>EKVIIEKAAGDAEAIAFDGRTYMEYHNAVTKSHLSNEIPAEKALQSNHFELSIKTEATQGLILWSGKGLERSDYIALAIVDGFVQMMYDLGSKPVVLRSTVPINTNHWTHIKAYRVQREGSLQVGNEAPITGSSPLGATQLDTDGALWLGGMERLSVAHKLPKAYSTGFIGCIRD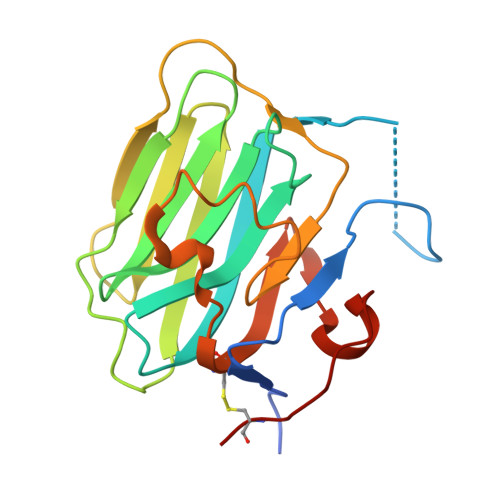VIVDRQELHLVEDALNNPTILHCSAK[2x]> MGSSHHHHHHSQD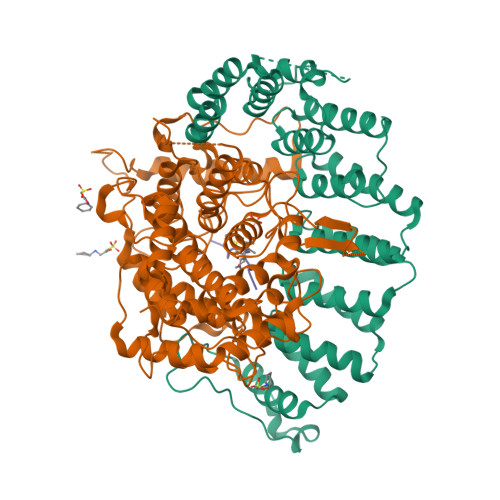LMVTSTYIPMSQRRSWADVKPIMQDDGPNPVVPIMYSEEYKDAMDYFRAIAAKEEKSERALELTEIIVRMNPAHYTVWQYRFSLLTSLNKSLEDELRLMNEFAVQNLKSYQVWHHRLLLLDRISPQDPVSEIEYIHGSLLPDPKNYHTWAYLHWLYSHFSTLGRISEAQWGSELDWCNEMLRVDGRNNSAWGWRWYLRVSRPGAETSSRSLQDELIYILKSIHLIPHNVSAWNYLRGFLKHFSLPLVPILPAILPYTASKLNPDIETVEAFGFPMPSDPLPEDTPLPVPLALEYLADSFIEQNRVDDAAKVFEKLSSEYDQMRAGYWEFRRRECAE;> MATEFTPSVYSLVSKPLPSNSRPSATLDEQAETEDLISQLFDLTADPNALVSEHGKRYSGLRKQEHTQFLASSFFQLPGKFVSLDASRPWLVFWTVHSLDLLGVALDQGTKDRVVSTLLHFLSPKGGFGGGPANSQIPHLLPTYASVCSLAIAGNDSSTGGWKDLAAARQSIYEFFMRCKRPDGGFVVCEGGEVDVRGTYCLLVVATLLDIITPELLHNVDKFVSACQTYEGGFACASFPFPSVVPSTSAFPTSEPSCRVSMAEAHGGYTSCSLNSHFLLTSVPLPSFPLSIDANAALRWTVLQQGEPIEGGGFRGRTNKLVDGCYSWWVGGGAPVAEELVRREKSRKVKKSRIEVFEEEKEGDWEDVPPIPPIFNRVALQEFTLVAAQQDPGSTGGLRDKPGKRPDQYHTCNNLSGLSIAQHKMSHSPSTVSSNRLKFDASKGLPAVKPVAPGGGWKNEDERQNARREIWANALGWIEEEGGEIIVGGKDNRINTTTPVFNILGLRLKPFINYFYCQEN;> DDPTASACNIQ>[4x]KFRPEMLQGKKVIVTGASKGIGREIAYHLAKMGAHVVVTARSKEALQKVVARCLELGAASAHYIAGSMEDMTFAEEFVAEAGNLMGGLDMLILNHVLYNRLTFFHGEIDNVRKSMEVNFHSFVVLSVAAMPMLMQSQGSIAVVSSVAGKITYPLIAPYSASKFALDGFFSTLRSEFLVNKVNVSITLCILGLIDTETAIKATSGIYLGPASPKEECA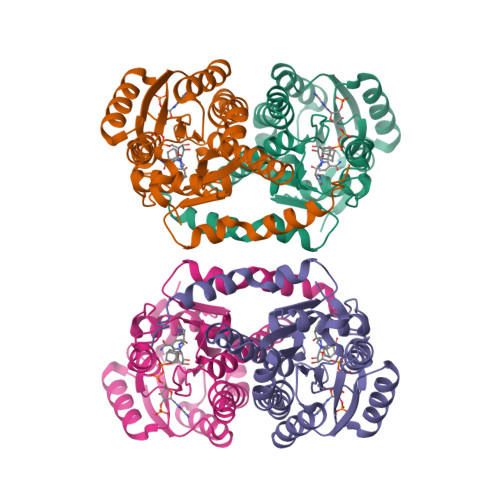LEIIKGTALRQDEMYYVGSRWVPYLLGNPGRKIMEFLSAAEYNWDN> SFWYGAM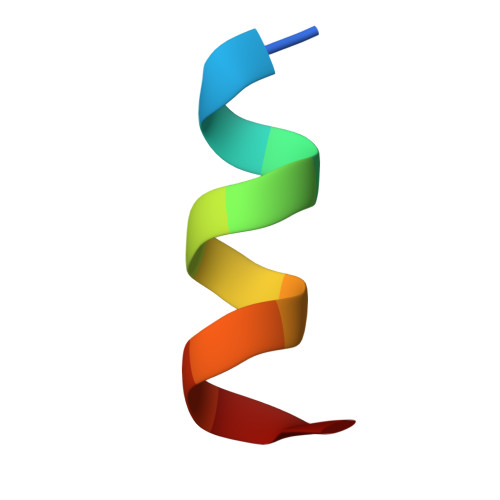KALYG Contractile bacteriophages of the family Myoviridae (i.e. T4), R-type pyocins and the type VI secretion system (T6SS) of Gram-negative bacteria are evolutionarily related nano-scale injection machines that puncture target cell membranes using a shared contraction mechanism. TssA subunits are enigmatic as they possess a conserved N-terminal region of unknown function, previously identified as ImpA_N (PFAM: PF0681226), whereas sequences located C-terminal to this region are highly divergent. Consistent with this, phylogenetic analysis has suggested that the TssA family can be subdivided into three clades (TssA1, TssA2 and TssA3). The structural studies presented here show that TssA1B, TssA2A and TssA2B possess structurally diverse CTDs that lead to distinct overall architectures for their respective complexes.

The structure of a Bc TssA1B CTD domain construct (I303-S373) was determined to 3.08 Å and the asymmetric unit was observed to contain eight CTD monomers (chains A–H). Each chain folds into four α-helices (α12-α15) that lie in approximately the same plane, and form two antiparallel pairs. The eight monomers in the asymmetric unit further assemble into a higher order oligomer of 32 subunits, consistent with the SEC-MALLS analysis of TssA1B and TssA1B CTD oligomers, with D16 symmetry using the crystallographic two-fold axes to make up a double-layered ring with 16 subunits in each layer. In the assembled Bc TssA1B CTD ring, analysis by PISA32 revealed an extensive dimer interface (~950 Å2) between monomers in the different layers, which principally involves the interaction of residues located in helices α12–α13 with their two-fold related subunits forming a region of hydrophobic packing with hydrophilic interactions at the periphery. Further less extensive interactions (~570 Å2) were identified between dimers that facilitate formation of the ring, with each pair of helices α14-α15 in one dimer, together with a small number of residues from α13, interacting with their equivalents in adjacent 16-fold related dimers on either side. This type of interlocking series of interactions is repeated in a cyclic arrangement to form a double-layered ring. In the crystal structure of the TssA1B CTD oligomer, the double ring is ~25 Å thick with a lumenal diameter of ~110 Å and an outer diameter of ~200 Å, in agreement with the dimensions of Bc TssA1B and purified CTD oligomers determined by negative stain EM analysis. The C-termini of the TssA1B CTD monomers are located at the inner face of the ring, while their N-termini are orientated on the outside, consistent with EM analysis, which places the Nt1 domain at the periphery of the ring in the intact complex. The Bc TssA1B CTD structure shows that this motif defines a loop that connects α12 and α13, and includes a salt bridge between E324 from this motif and a conserved arginine, R306, from a symmetry-related subunit.

>[8x]ISHMIQNRAQAVDQLRAVARYFRQTEPHSPVAYLADKAAEWADMPLHKWLESVVKDDGSLSHIRELLGVRPDEQS> MKFALQINEGPYQHQASDSAYQFAKAALEKGHEIFRVFFYHDGVNNSTRLTTPPQDDRHIVNRWAELAEQYELDMVVCVAAAQRRGIVDEGEASRNGKDATNIHPKFRISGLGQLVEAAIQADRL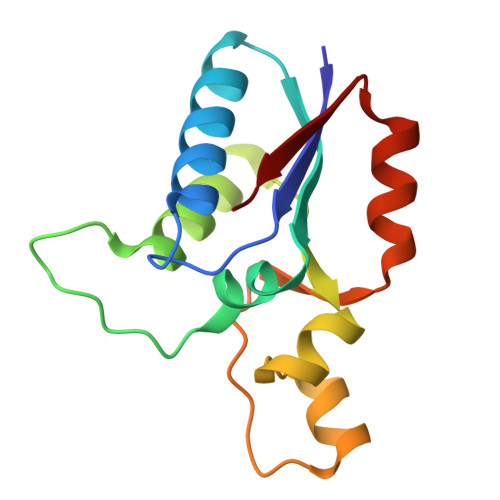VVFGD Kinesins are a family of microtubule-based motors that play important roles in intracellular transport and cell division. Kinesin-1 transports cargo within cells, a process tightly coupled with ATP hydrolysis. Whereas kinesin-1 in solution is mostly loaded with ADP, ADP release is accelerated several thousand-fold upon microtubule binding. Here we characterized kinesin-1 P-loop mutations that interfere with ADP binding and determined the structure of the corresponding mutated nucleotide-free kinesins.

Using these T87A crystals as seeds, we were also able to crystallize wild-type apo-kinesin-1 and the T92V mutant and to determine their structures. Whereas most of the following analysis was performed taking the apo-T87A structure as a reference, identical conclusions could be reached from these wild-type apo-kinesin and T92V isomorphous structures. Taken together, these observations suggest that the P-loop destabilization in nucleotide-free T87A, as well as in the isomorphous structure of wild-type apo-kinesin and of T92V, is the combined result of ADP release and of the loss of the T87-E236 interactions. Whereas we demonstrated that, in the absence of microtubules, apo-kinesin-1 may adopt two conformations, ADP-kinesin-like and tubulin-bound apo-kinesin-like, the effect of tubulin binding is to shift the balance between them and to stabilize the tubulin-bound apo-kinesin-like conformation, from which ADP is released and which is primed to bind ATP6.

>MADLAESNIKVMCRFRPLNESEVNRGDKYIAKFQGEDTVVIASKPYAFDRVFQSSTSQEQVYNDAAKKIVKDVLEGYNGTIFAYGQTSSGKTHTMEGKLHDPEGMGIIPRIVQDIFNYIYSMDENLEFHIKVSYFEIYLDKIRDLLDVSKTNLSVHEDKNRVPYVKGATERFVSSPDEVMDTIDEGKSNRHVAVTNMNEHSSRSHSIFLINVKQENTQTEQKLSGKLYLVDLAGSEKVSKTGAEGAVLDEAKNINKSLSALGNVISALAEGSTYVPYRDSKMTRILQDSLGGNARTTIVICCSPSSYNESETKSTLLFGQRAKTI[6x]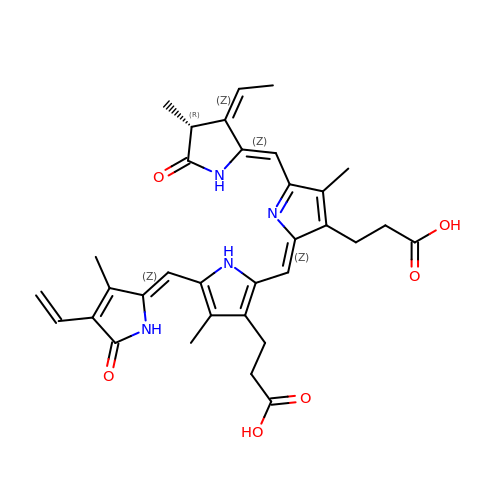3-[5-[(~{Z})-(4-ethenyl-3-methyl-5-oxidanylidene-pyrrol-2-ylidene)methyl]-2-[(~{Z})-[5-[(~{Z})-[(4~{R})-3-ethyl-4-methyl-5-oxidanylidene-pyrrolidin-2-ylidene]methyl]-3-(3-hydroxy-3-oxopropyl)-4-methyl-pyrrol-2-ylidene]methyl]-4-methyl-1~{H}-pyrrol-3-yl]propanoic acid | C33 H36 N4 O6 | SNHIGJASYQUMKZ-NSNBCYBJSA-N> ACDYTCGSNCYSSSDVSTAQAAGYKLHEDGETVGSNSYPHKYNNWEGFDF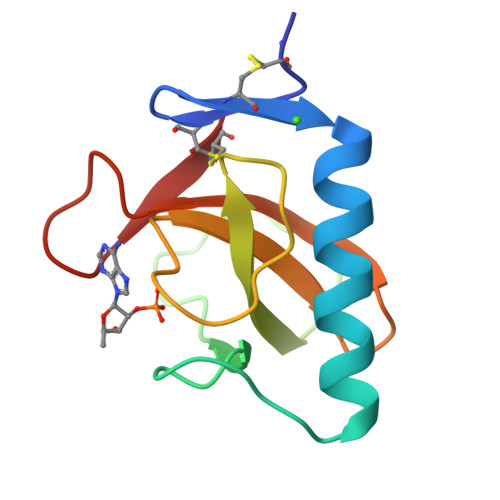SVSSPYYEWPILSSGDVYSGGSPGADRVVFNENNQLAGVITHTGASGNNFVECT> MRSRRVDVMDVMNRLILAMDLMNRDDALRVTGEVREYIDTVAIGYPLVLSEGMDIIAEFR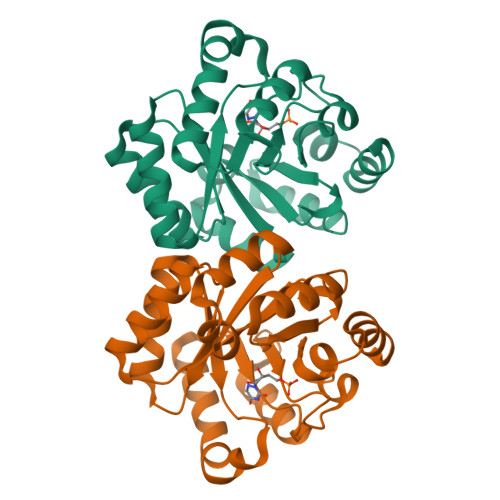KRFGCRIIADFKVADIPETNEKICRATFKAGADAIIVHGFPGADSVRACLNVAEEMGREVFLLTEMSHPGAEMFIQGAADEIARMGVDLGVKNYVGPSTRPERLSRLREIIGQDSFLISPGVGAQGGDPGETLRFADAIIVGRSIYLADNPAAAAAGIIESIKDLLIPEDPAANKARKEAELAAATA> TTHFTVTDQWGNVVSYTTTIEQLFGTGILVPGYGLFLNNELTDFDAIPGGANEVQPNKRPLSSMTPTIVFKDEKPVLTVGSPGGTTIIASVFQTILNYFEYGMSLQDAIEE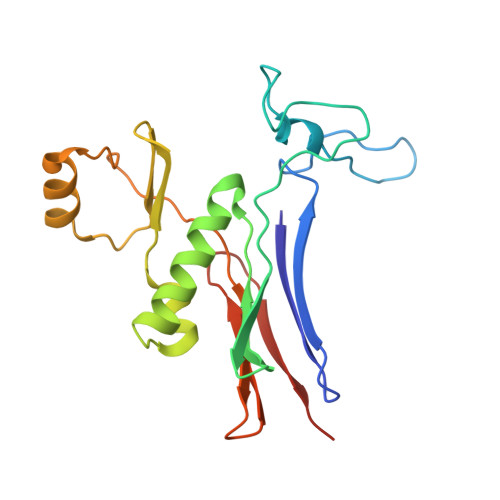PRIYTNSLTSYRYESGMPEDVRRKLNDFGHKFGSNPVDIGNVQSIFIDRENKTFMGVADSSRNGTAVGVNIKTSAK> KPQVTILATGGTIAGAVTVDKLLAAVPAINDLATIKGEQISSIGSQEMTGKVWLKLAKRVNELLAQKETEAVIITHGTDTMEETAFFLNLTVKSQKPVVLVGAMRPGSSMSADGPMNLYNAVNVAINKASTNKGVVIVMNDEIHAAREATKLNTTAVNAFASPNTGKIGTVYYGKV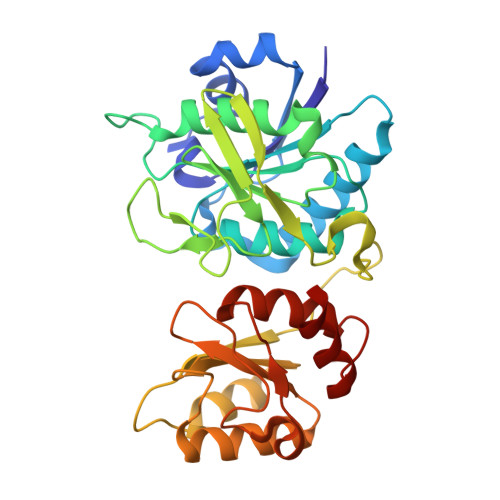EYFTQSVRPHTLASEFDISKIEELPRVDILYAHPDDTDVLVNAALQAGAKGIIHAGMGNGNPFPLTQNALEKAAKSGVVVARSSRVGSGSTTQEAEVDDKKLGFVATESLNPQKARVLLMLALTKTSDREAIQKIFSTY>[2x]ANPLYQKHIISINDLSRDDLNLVLATAAKLKANPQPELLKHKVIASCFFAASTRTRLSFETSMHRLGASVVGFSDSANTSLGKKGETLADTISVISTYVDAIVMRHPQEG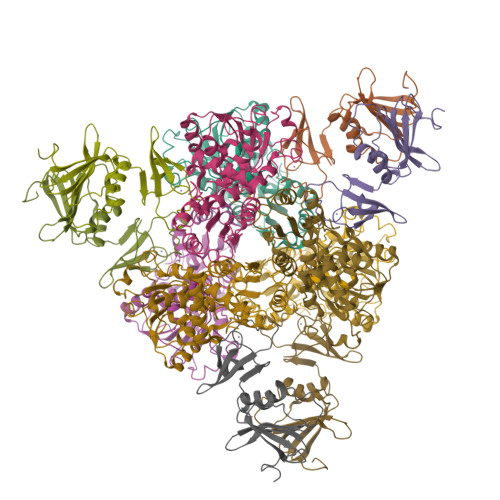AARLATEFSGNVPVLNAGDGSNQHPTQTLLDLFTIQETQGRLDNLHVAMVGDLKYGRTVHSLTQALAKFDGNRFYFIAPDALAMPQYILDMLDEKGIAWSLHSSIEEVMAEVDILYMTRVQKERLDPSEYANVKAQFVLRASDLHNAKANMKVLHPLPRVDEIATDVDKTPHAWYFQQAGNGIFARQALLALVLNRDLVL;>MTHDNKLQVEAIKRGTVIDHIPAQIGFKLLSLFKLTETDQRITIGLNLPSGEMGRKDLIKIENTFLSEDQVDQLALYAPQATVNRIDNYEVVGKSRPSLPERIDNVLVCPNSNCISHAEPVSSSFAVRKRANDIALKCKYCEKEFSHNVVLAN[2x]> MLTSAGIAMGQASKLAAATKAAEQTGLKSAYKDNFLIGAALNATIASGADERLNTLIAKEFNSITPENCMKWGVLRDAQGQWNWKDADAFVAFGTKHNLHMVGHTLVWHSQIHDEVFKNADGSYISKAALQKKMEEHITTLAGRYKGKLAAWDVVNEAVGDDLKMRDSHWYKIMGDDFIYNAFTLANEVDPKAHLMYNDYNIERTGKREATVEMIERLQKRGMPIHGLGIQGHLGIDTPPIAEIEKSIIAFAKLGLRVHFTSLDVDVLP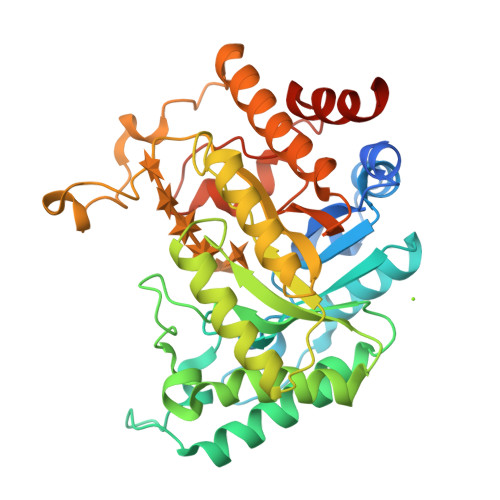SVWELPVAEVSTRFEYKPERDPYTKGLPQEMQDKLAKRYEDLFKLFIKHSDKIDRATFWGVSDDASWLNGFPIPGRTNYPLLFDRKLQPKDAYFRLLDLKRLEHHHHHH> NNKTLAAMKNFAEQYAKRTDTYFCSDLSVTAVVIEGLARHKEELGSPLCPCRHYEDKEAEVKNTFWNCPCVPMRERKECHCMLFLTPDNDFAGDAQDIPMETLEEVKAS;> MNVGDRVRVTSSVVVYHHPEHKKTAFDLQGMEGEVAAVLTEWQGRPISANLPVLVKFEQR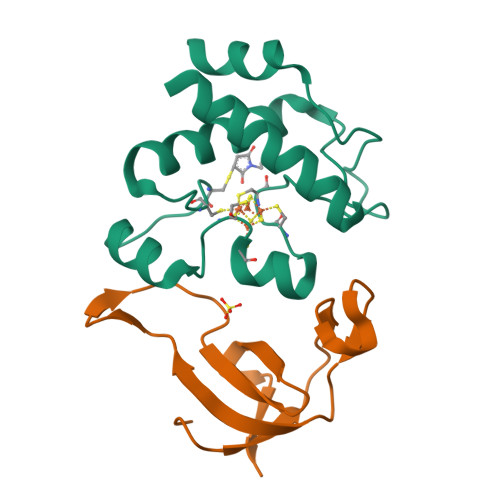FKAHFRPDEVTLI> PLSEIPTDDNPNMSMAEMLRRDEGLRLKVYWDTEGYPTIGIGHLIMKQPVRDMAQINKVLSKQVGREITGNPGSITMEEATTLFERDLADMQRDIKSHSKVGPVWQAVNRSRQMALENMAFQMGVGGVAKFNTMLTAMLAGDWEKAYKAGRDSLWYQQTKGRASRVTMIILTG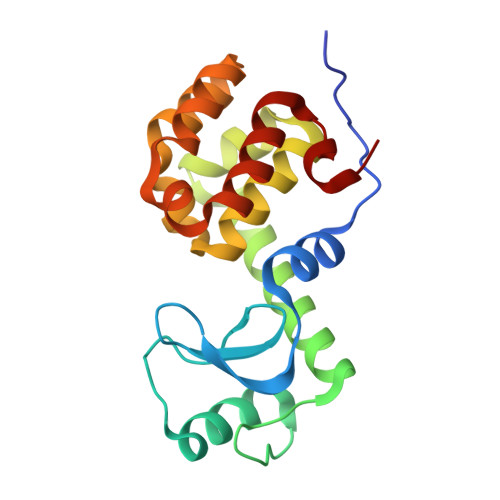NLESYGVE>[2x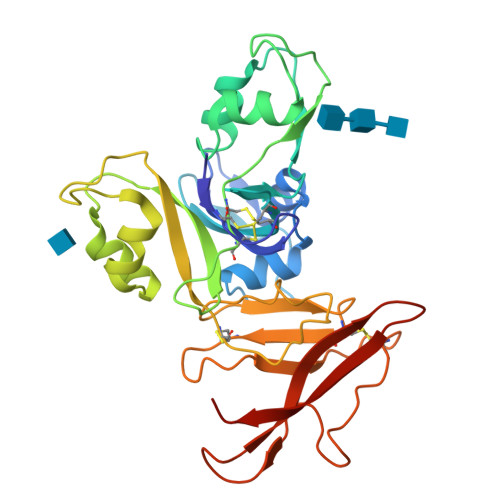]ANFTCAVASGTTCKSAILYTSPNATTYGNLVARFNTTTLPDLLGANGLPDGTLSSAPVAANSTVKIPFRCRCNGDVGQSDRLPIYVVQPQDGLDAIARNVFNAFVTYQEIAAANNIPDPNKINVSQTLWIPLPCSCDKEEGSNVMHLAYSVGKGENTSAIAAKYGVTESTLLTRNKIDDPTKLQMGQILDVPLPVCRSSISDTSADHNLMLLPDGTYGFTAGNCIRCSCSSTTYQLNCTAVQNKGCPSVPLCNGTLKLGETNGTGCGSTTCAYSGYSNSSSLIIQTSLATNQTTACQ> GSSHHHHHHSSGENLYFQHMKTAQEFRAGQVANINGAPWVIQKAEFNKSGRNAAVVKMKLKNLLTGAGTETVFKADDKLEPIILDRKEVTYSYFADPLYVFMDSEFNQYEIEKDDLEGVLTFIEDGMTDICEAVF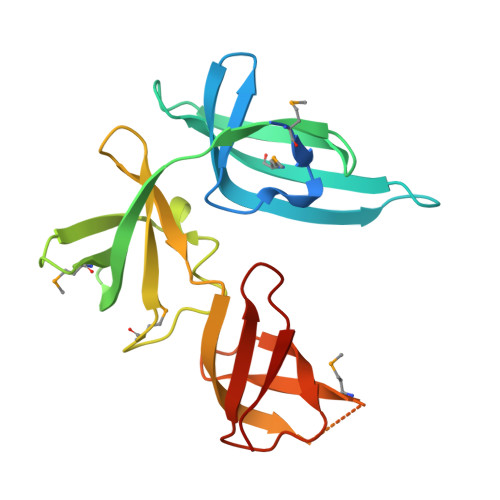YNDKVISVELPTTIVRQIAYTEPAVRGDTSGKVMKTARLNNGAELQVSAFCEIGDSIEIDTRTGEYKSRVKA N,N'-(furan-2,5-diylbis{benzene-4,1-diyl[(Z)-aminomethylylidene]})diethanaminium | C22 H26 N4 O | 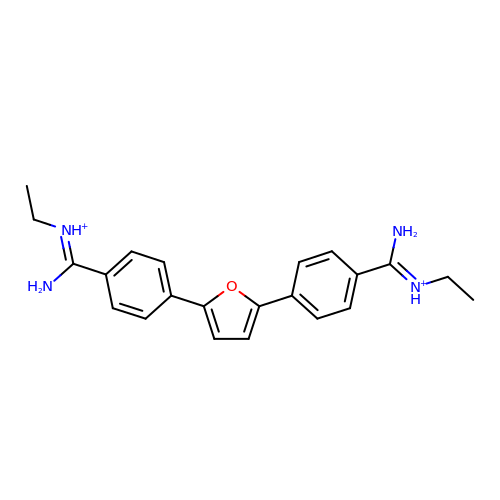UDRBFQQQLONWPG-UHFFFAOYSA-P> ASGSGQSTRYWDCCKPSCAWPGKAAVSQPVYACDANFQRLSDFNVQSGCNGGSAYSCADQTPWAVNDNLAYGFAATSIAGGSESSWCCACYALTF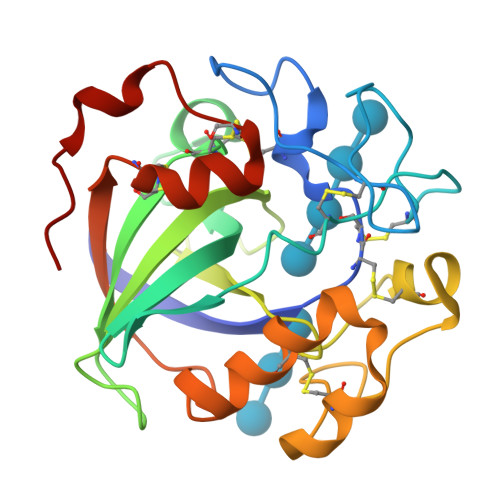TSGPVAGKTMVVQSTSTGGDLGSNQFDIAMPGGGVGIFNGCSSQFGGLPGAQYGGISSRDQCDSFPAPLKPGCQWRFDWFQNADNPTFTFQQVQCPAEIVARSGCKRNDDSSFPVFTP4-(3-amino-1H-pyrazol-4-yl)phenol 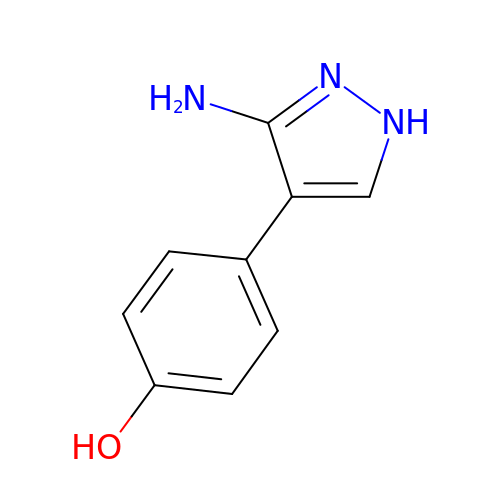| C9 H9 N3 O | WRERTDQKTDJJIZ-UHFFFAOYSA-N N-{4-[1-(2-FLUOROBENZYL)-3-BUTYL-2,6-DIOXO-2,3,6,7-TETRAHYDRO-1H-PURIN-8-YLMETHYL]-PHENYL}-ACETAMIDE | C25 H26 F N5 O3 | 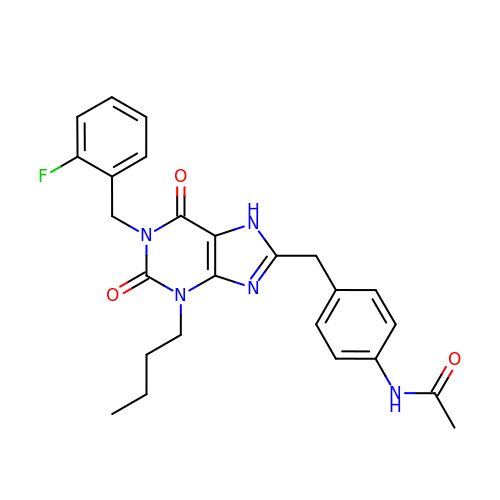JHSHXKJSPVHPCJ-UHFFFAOYSA-N2-amino-2-deoxy-beta-D-glucopyranuronic 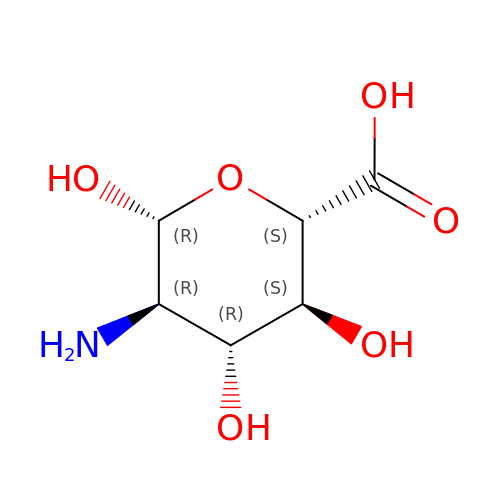acid | C6 H11 N O6 | CRIPFXSBMSGPKB-LVBGKUAWSA-N> MTTITTTTNNTFDLANVIAEYKAGFEQYKADNKQYNADAYRRKIES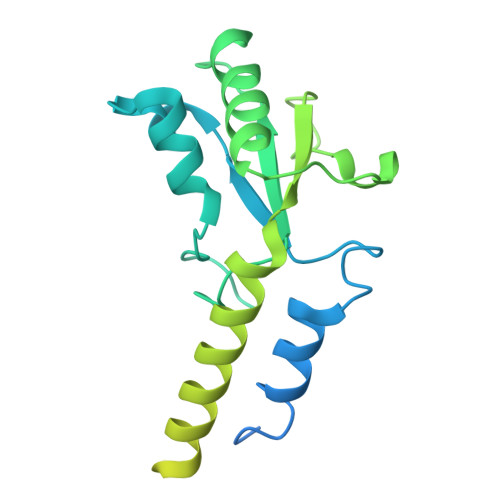INSDAALTNGAFNQFAYGSQMFEGKTLQEIAESLKTMQVKDSSREDENGLIFPHVTLQLVSPTTPAQYYGLIAEAVKLGFEVCPDWRLHVGTGRNFPACRLVRQAEWYKPHNEKLMAERIAEAEKQEAERLKAEYFNEHRVQAYVEQAQRKFMATQAQQAAISLSAAISRELYASSGLSDDDLAVVAQSDVWAFNTLAPQLQEKDPNVISAALTGAGFVKGKHKLSDGKQATLWVKDGADVTALTLESKYIQ>GSMAFLILVIGNLHIPDRALDIPPKFKKLLSPGKISQTLCLGNLTDRATYDYLRSISPDLKIVRGRMDVEATSLPLMQVVTHGSLRIGFLEGFTLVSEEPDVLLAEANKLDVDVLCWAGGSHRFECFEYMDKFFVNPGSATGAFTTDWLAEGEEV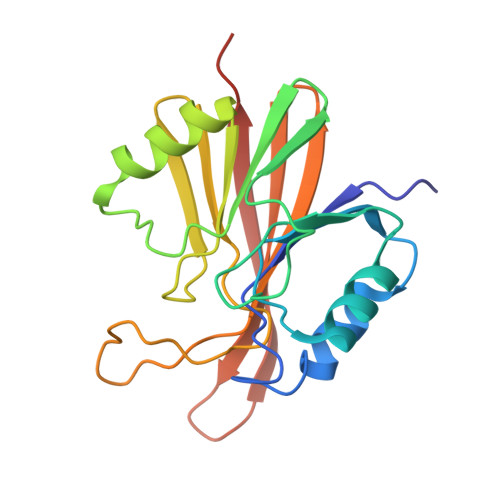VPSFCLMDVQGISLTLYVYQLRKDENGTENVAVEKVTYTKPVEPTGAS[6x]> HPNSPLDEENLTQENQDRGTHVDLGLASANVDFAFSLYKQLVLKAPDKNVIFSPLSISTALAFLSLGAHNTTLTEILKGLKFNLTETSEAEIHQSFQHLLRTLNQSSDELQLSMGNAMFVKEQLSLLDRFTEDAKRLYGSEAFATDFQDSAAAKKLINDYVKNGTRGKITDLIKDLDSQTMMVLVNYIFFKAKWEMPFDPQDTHQSRFYLSKKKWVMVPMMSLHHLTIPYFRDEELSCTVVELKYTGNASALFILPDQDKMEEVEAMLLPETLKRWRDSLEFREIGELYLPKFSISRDYNLNDILLQLGIEEAFTSKADLSGITGARNLAVSQVVHKA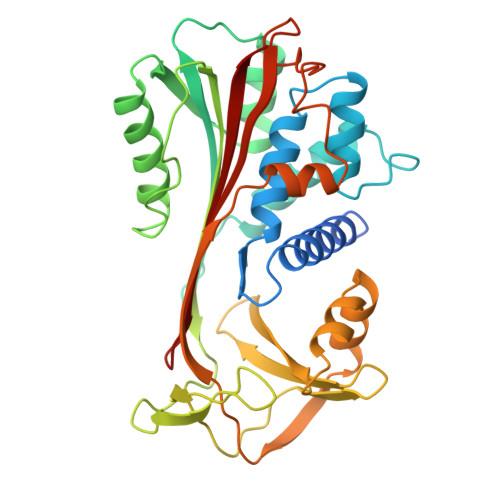VLDVFEEGTEASAATAVKITLL> SMADPQTDTIAALIADVAKANQRLQDLSDEVQAEQESVNKAMVDVETARDNAAAAEDDL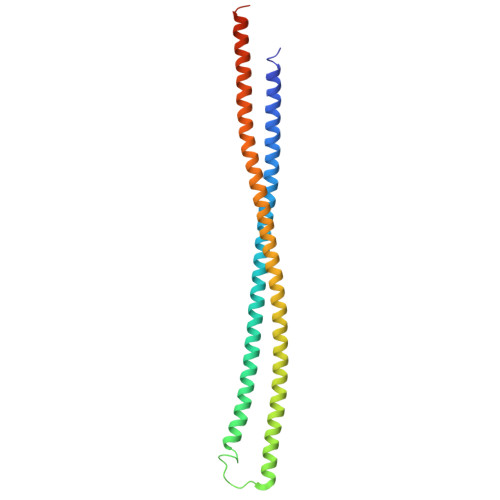EVSQRAVKDANAAIAAAQHRFDTFAAATYMNGPSVSYLSASSPDEIIATVTAAKTLSASSQAVMANLQRARTERVNTESAARLAKQKADKAAADAKASQDAAVAALTETRRKFDEQREEVQRLAAERDAAQARLQAARLVAWSSEGGQGAPPFRMWDPGS(2~{R},3~{R},4~{R},5~{S})-1-[5-[[4-(3,4-dihydro-2~{H}-1,5-benzodioxepin-7-yl)phenyl]methoxy]pentyl]-2-(hydroxymethyl)piperidine-3,4,5-triol 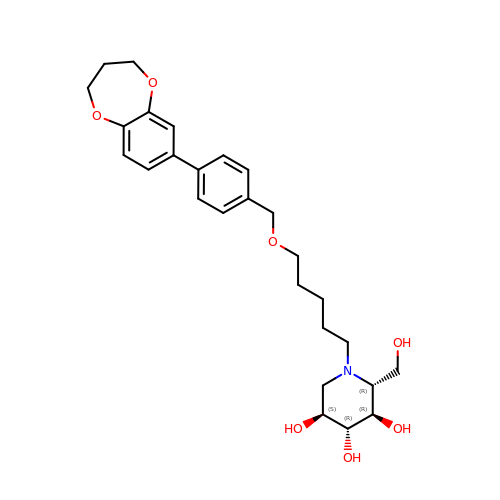| C27 H37 N O7 | FGUXCOMLHUOVQN-QGNCETNGSA-N> RGSFVEMVDNLRGKSGQGYYVEMTVGSPPQTLNILVDTGSSNFAVGAAPHPFLHRYYQ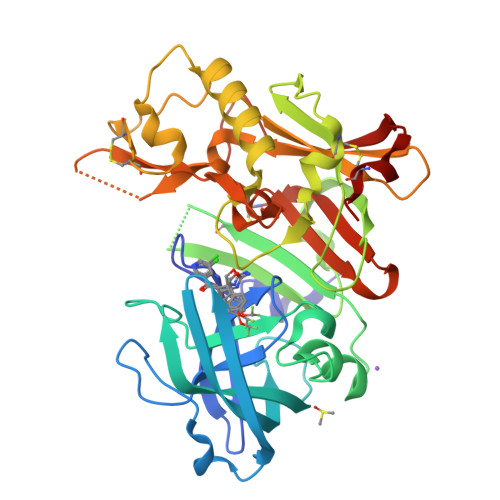RQLSSTYRDLRKGVYVPYTQGKWEGELGTDLVSIPHGPNVTVRANIAAITESDKFFINGSNWEGILGLAYAEIARPDDSLEPFFDSLVKQTHVPNLFSLQLCGAGFPLNQSEVLASVGGSMIIGGIDHSLYTGSLWYTPIRREWYYEVIIVRVEINGQDLKMDCKEYNYDKSIVDSGTTNLRLPKKVFEAAVASIKAASSTEKFPDGFWLGEQLVCWQAGTTPWNIFPVISLYLMGEVTNQSFRITILPQQYLRPVEDVATSQDDCYKFAISQSSTGTVMGAVIMEGFYVVFDRARKRIGFAVSACHVHDEFRTAAVEGPFVTLDMEDCGYN Colonization of these different niches involves an N-acetylglucosamine binding protein (GbpA) that has been reported to mediate bacterial attachment to both marine chitin and mammalian intestinal mucin through an unknown molecular mechanism. Recent studies have suggested that Vibrio cholerae secretes a protein that mediates adhesion in aquatic environments, e.g. to plankton, as well as adhesion to human intestinal cells. This protein, GlcNAc binding protein A (GbpA) binds to N-acetylglucosamine (GlcNAc)- containing carbohydrates, such as chitin, and is secreted by the type 2 secretion system. We report structural studies that reveal that GbpA possesses an unusual, elongated, four-domain structure, with domains 1 and 4 showing structural homology to chitin binding domains. Finally, mouse virulence assays show that only the first three domains of GbpA are required for colonization. These results explain how GbpA provides structural/functional modular interactions between V. cholerae, intestinal epithelium and chitinous exoskeletons.

Although extensive efforts were made to crystallise full-length GbpA, GbpAD1–3 was the longest construct that could be crystallised. The GbpAD1–3 structure was solved by SAD phasing, and refined against 1.8 Å synchrotron diffraction data. The structure of GbpAD1–3 reveals three distinct domains rich in β-structure, linked by disordered loops. Domain 1 (GbpAD1) comprises a four-stranded and a three-stranded β-sheet forming a β-sandwich. Between β-strands 1 and 3, a 65-residue loop forms a pseudo-domain, which consists of short α-helices, a β-strand, and loops. There are also two disulphide bonds formed: one in the loop/helical region (Cys-42 and Cys-56) and one linking β-strands 4 and 5 (Cys-152 and Cys-169). A structural similarity search with the Dali server identified chitin binding protein 21 (CBP21) from S. marcescens, which is part of the CAZy Carbohydrate Binding Module family 33 (CBM33) as a structural homologue (RMSD = 0.9 Å for 168 Cαatoms, 47% sequence identity). Structural similarity searches with DALI revealed only distant structural similarities between domain 2 of GbpA and the β-domain of the flagellin protein p5 (Z = 4.0, RMSD = 2.9 Å for 68 Cα atoms). A more significant structural match was observed for domain 3 of GbpA. This domain has an immunoglobulin fold with significant structural similarity to over 200 structures in the PDB. The crystal structure of GbpAD1–3 lacks the C-terminal domain 4, comprising residues 415–485.

>[2x]HGYVSAVENGVAEGRVTLCKFAANGTGEKNTHCGAIQYEPQSVEGPDGFPVTGPRDGKIASAESALAAALDEQTADRWVKRPIQAGPQTFEWTFTANHVTKDWKYYITKPNWNPNQPLSRDAFDLNPFCVVEGNMVQPPKRVSHECIVPEREGYQVILAVWDVGDTAASFYNVIDVKFDGNGPVLPDWNPAGQIIPSMDLSIGDTVYTRVFDNDGENPAYRTELKIDSETLTKANQWSYALATKINQTQKQQRAGQLNGDQFVPVYGTNPIYLKEGSGLKSVEIGYQIEAPQPEYSLTVSGLAKEYEIGEQPIQLDLTLEAQGEMSAELTVYNHHQKPLASWSQAMTDGELKSITLELSEAKAGHHMLVSRIKDRDGNLQDQQTLDFMLVE>[12x]HVKSGLQIKKNAIIDDYKVTSQVLGLGINGKVLQIFN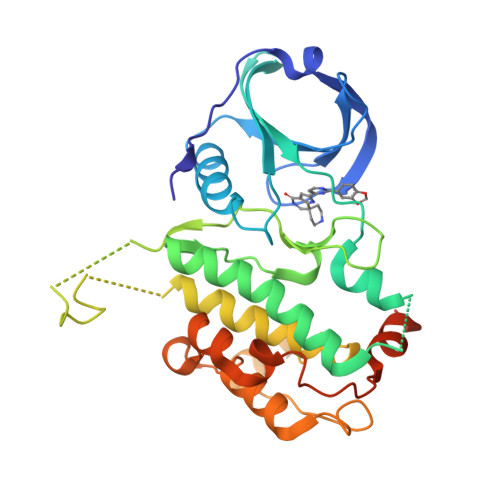KRTQEKFALKMLQDCPKARREVELHWRASQCPHIVRIVDVYENLYAGRKCLLIVMECLDGGELFSRIQDRGDQAFTEREASEIMKSIGEAIQYLHSINIAHRDVKPENLLYTSKRPNAILKLTDFGFAKETTSHNSLTTPCYTPYYVAPEVLGPEKYDKSCDMWSLGVIMYILLCGYPPFYSNHGLAISPGMKTRIRMGQYEFPNPEWSEVSEEVKMLIRNLLKTEPTQRMTITEFMNHPWIMQSTKVPQTPLHTSRVLKEDKERWEDVKEEMTSALATMR>[2x]MSEELVPHPNESLPGPRASPREVWKKGGRLLSVLLAVNVLLLACTLISGGAFNKVAVYDTDVFALLTTMMLLAALWIVFYLLRTARCPDAVPYRDAHAGPIWLRGGLVLFGICTLVMDVFKTGYYSSFFECQSAIKILHPIIQAVFVIVQTYFLWISAKDCIHTHLDLTRCGLMFTLATNLAIWMAAVVDESVHQAHSYSGSHGNTSHTRLNPDSKRAGGAAEEDPCLCSTAICQIFQQGYFYLYPFNIEYSLFASTMLYVMWKNVGRLLASTHGHGHTPSRVSLFRETFFAGPVLGLLLFVVGLAVFILYEVQVSGERGHTRQALVIYYSFNIVCLGLMTLVSLSGSVIYRFDRRAMDHHKNPTRTLDVALLMGAALGQYAISYYSIVAVVVGSPRDLQGALNLSHALLMIAQHTFQNVFIIESLHRGPPGAEPREMPPKEPCQGITFANLDAIRTLPSCPPTPRLVIPNLESPQEAVAIISAPRCHWRRRCLKDISLFLLLCNVILWIMPAFGARPHFSNTVEVDFYGYSLWAAIVNICLPFGIFYRMHAVSSLLEVYVLS

The otopetrin (OTOP) proteins were recently characterized as extracellular proton-activated proton channels. Several recent OTOP channel structures demonstrated that the channels form a dimer with each subunit adopting a double-barrel architecture. In this study, we performed structural and functional characterization of the Caenorhabditis elegans OTOP8 (CeOTOP8) and mouse OTOP2 (mOTOP2) and illuminated a set of conformational changes related to the proton-conducting process in OTOP. Combining the structural information from both channels, we propose a working model describing the multi-step conformational changes during the proton conducting process.

Mouse OTOP2 was expressed in HEK293F cells and purified in glyco-diosgenin (GDN) detergent. Its single-particle cryo-EM structures were determined using protein samples prepared at various pH conditions (5.0, 7.0, 8.0, and 9.0). The mOTOP2 structures at pH 8.0 and 9.0 are virtually identical. Among all, the mOTOP2 structures determined at pH 5.0 and 8.0 are better resolved and will be used to represent the low and high pH structures, respectively, in the following discussion. The structure difference in mOTOP2 between low and high pH conditions is quite subtle and mainly occurs at the N-terminal half of TM6 preceding the highly conserved glutamate (Glu250 in mOTOP2) important for proton transfer. At higher pH, however, the N-terminal half of the TM6 helix unwinds to an extended loop (right insets). This helix-to-loop structural transition occurs before the conserved Pro246 and vacates the space above Glu250 initially occupied by Pro246, allowing the Glu250 side chain to flip upwards and become completely exposed to the external solution. The outward-facing Glu250 is also stabilized by forming an H-bond with Tyr245 and a salt bridge with Arg517 in the high pH mOTOP2 structure. In state 1, a loop configuration at the N-terminal part of TM6 allows the glutamate to be exposed to the extracellular solution for protonation. The two conformations observed in mOTOP2 structures represent these first two states of the proton-conducting process, whereas the CeOTOP8 structures likely capture the next two states (states 3 and 4).> MSDNRRRRREEDDSDSENELPPSSPQQHFRGGMNPVSSPIGSPDMINPEGDDNEVDDVPDIDEVEEQMNEVDLMDDNMYEDYAADHNRDRYDPDQVDDREQQELSLSERRRIDAQLNERDRLLRNVAYIDDEDEEQEGAAQLDEMGLPVQRRRRRRQYEDLENSDDDLLSDMDIDPLREELTLESLSNVKANSYSEWITQPNVSRTIARELKSFLLEYTDETGRSVYGARIRTLGEMNSESLEVNYRHLAESKAILALFLAKCPEEMLKIFDLVAMEATELHYPDYARIHSEIHVRISDFPTIYSLRELRESNLSSLVRVTGVVTRRTGVFPQLKYVKFNCLKCGSILGPFFQDSNEEIRISFCTNCKSKGPFRVNGEKTVYRNYQRVTLQEAPGTVPPGRLPRHREVILLADLVDVSKPGEEVEVTGIYKNNYDGNLNAKNGFPVFATIIEANSIKRREGNTANEGEEGLDVFSWTEEEEREFRKISRDRGIIDKIISSMAPSIYGHRDIKTAVACSLFGGVPKNVNGKHSIRGDINVLLLGDPGTAKS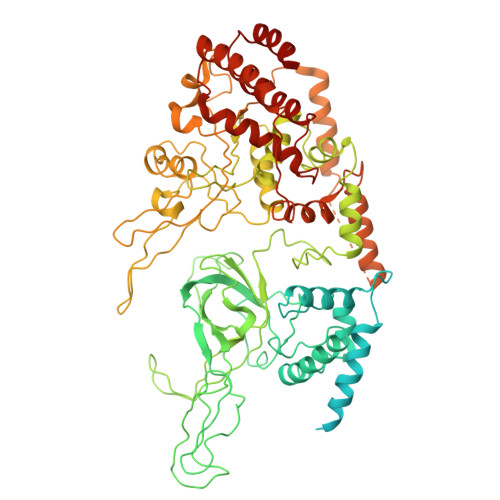QILKYVEKTAHRAVFATGQGASAVGLTASVRKDPITKEWTLEGGALVLADKGVCLIDEFDKMNDQDRTSIHEAMEQQSISISKAGIVTTLQARCSIIAAANPNGGRYNSTLPLAQNVSLTEPILSRFDILCVVRDLVDEEADERLATFVVDSHVRSHPENDEDREGEELKNNGESAIEQGEDEINEQLNARQRRLQRQRKKEEEISPIPQELLMKYIHYARTKIYPKLHQMDMDKVSRVYADLRRESISTGSFPITVRHLESILRIAESFAKMRLSEFVSSYDLDRAIKVVVDSFVDAQKVSVRRQLRRSFAIYTLGH> MGVLRIGHASLKVMDMDAAVRHYENVLGMKTTMKDKAGNVYLKCWDEWDKYSVILTPSDQAGMNHLAYKVEKEADLEALQQKIEAWGVKTTMLDEGTLPSTGRMLQFKLPSGHEMRLYASKEFVGTDVGNINPDPWPDGLK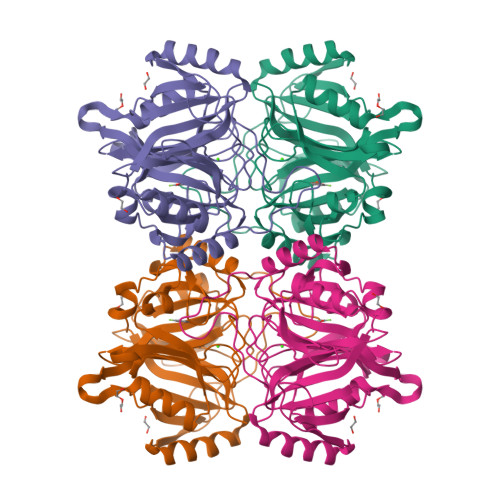GAGAHWLDHCLLVCEMNPEAGINTVADNTRFVTECLDFFLTEQVLVGPGGSIQATTFLARTTTPHDIAFVGGPTSGLHHIAFFLDSWHDVLKAADVMAKNKVRIDVAPTRHGITRGETIYFFDPSGNRNETFAGLGYLAQRDRPVTTWTEDQLGSAIFYHTGYLEPSFTDVYT>HMKICITVGHSILKSGACTSADGVVNEYQYNKSLAPVLADTFRKEGHKVDVIICPEKQFKTKNEEKSYKIPRVNSGGYDLLIELHLNASNGQGKGSEVLYYSNKGLEYATRICDKLGTVFKNRGAKLDKRLYILNSSKPTAVLIESFFCDNKEDYDKAKKLGHEGIAKLIVEGVLNKNI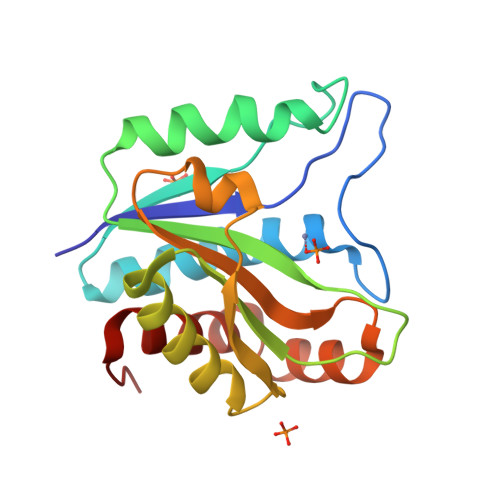N[4x]>MHHHHHHSSGRENLYFQGDVEYRPLTLNA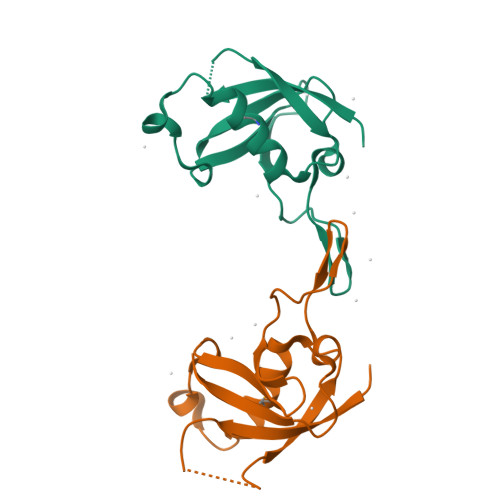LLAVGPGAGEAQGVPVKVLDCDTISQAKEKMLDQLYKGVPLTQRPDPRTLDVEWRSGVAGHLILSDEDVTSEVQGLWRRLNTLQHYKVPDGATVALVPCLTKHVLRENQ[2x]>[2x]MDNNKAEADTSSSMADPETRPTYTTHHLAIPSGVTQDEFDELKQSVVEFHT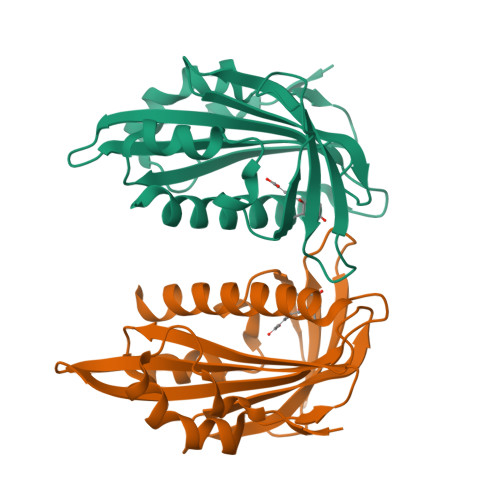YQLSQNQCSSLLAQRIRAPNDVVWSIVRRFDQPQTYKHFIKSCSVSDNFTMAVGSTRDVNVISGLPAATSTERLDILDDDRQVTGFSIIGGEHRLRNYRSVTSVHGFNRDGAICTVVLESYVVDVPEGNTEEDTRLFADTVVKLNLQKLVSVAESQVI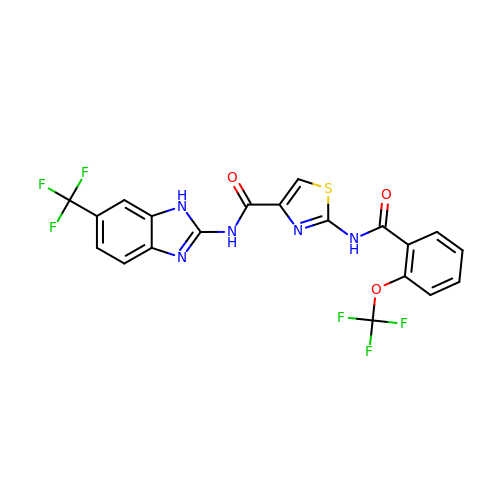2-{[2-(trifluoromethoxy)benzoyl]amino}-N-[6-(trifluoromethyl)-1H-benzimidazol-2-yl]-1,3-thiazole-4-carboxamide | C20 H11 F6 N5 O3 S | GUWQZSKMUJFZMM-UHFFFAOYSA-N> MARAAFLFKTVGFGGLQNVPINDELSSHLLRAGNSPWQLTQFLDWISLGRGLATSALVPTAGSRYYQMSCLLSGTLQIPFRPNHRWGDIRFLRLVWSAPTLDGLVVAPPQVLAQPALQAQADRVYDCDDYPFLARDPRFKHRVYQQLSAVTLLNLTGFGPISYVRVDEDMWSGDVNQLLMNYFGHTFAEIAYTLCQASANRPWEHDGTYARMTQIILSLFWLSYVGVIHQQNTYRTFYFQCNRRGDAAEVWILSCSLNHSAQIRPGNRSLFVMPTSPDWNMDVNLILSSTLTGCLCSGSQLPLIDNNSVPAVSRNIHGWTGRAGNQLHGFQVRRMVTEFCDRLRRDGVMTQAQQNQIE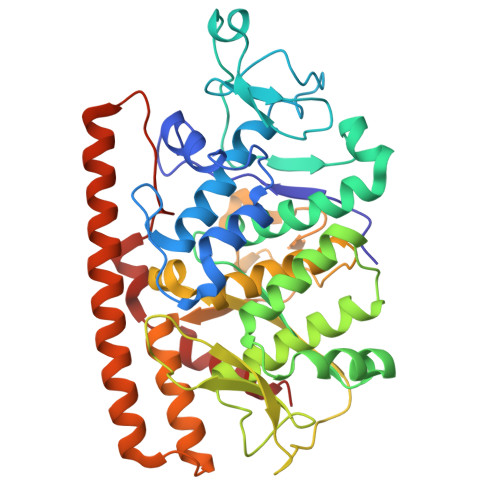ALADQTQQFKRDKLEAWAREDDQYNQANPNSTMFRTKPFTNAQWGRGNTGATSAAIAALI4-fluoro-N-{1-[5-(2-methylpyrimidin-4-yl)-5,6,7,8-tetrahydro-1,5-naphthyridin-2-yl]cyclopropyl}benzamide 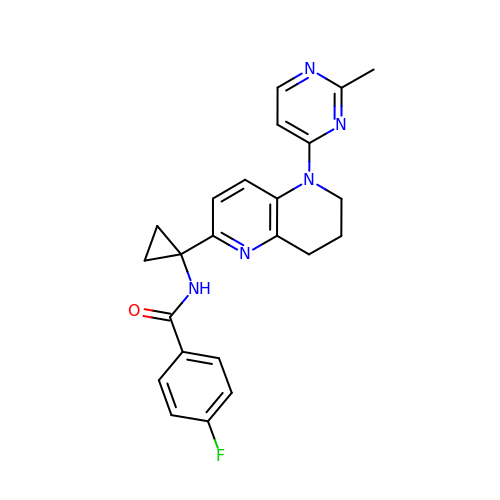| C23 H22 F N5 O | KKAMMYSFTPLTDH-UHFFFAOYSA-N> PAPHGGILQDLIARDALKKNELLSEAQSSDILVWNLTPRQLCDIELILNGGFSPLTGFLNENDYSSVVTDSRLADGTLWTIPITLDVDEAFANQIKPDTRIALFQDDEIPIAILTVQDVYKPNKTIEAEKVFRGDPEHPAISYLFNVAGDYYVGGSLEAIQLPQHYDYPGLRKTPAQLRLEFQSRQWDRVVAFQTRNPMHRAHRELTVRAAREANAKVLIHPVVGLTKPGDIDHHTRVRVYQEIIKRYPNGIAFLSLLPLAMRMSGDREAVWHAIIR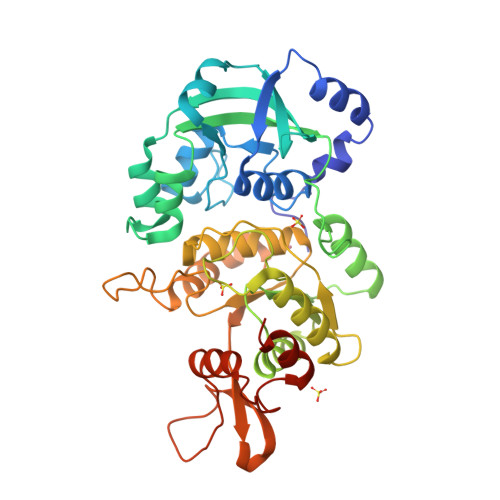KNYGASHFIVGRDHAGPGKNSKGVDFYGPYDAQELVESYKHELDIEVVPFRMVTYLPDEDRYAPIDQIDTTKTRTLNISGTELRRRLRVGGEIPEWFSYPEVVKILRESNPPRPKGSS>[2x]GPVHINKGGRPRQHLLSLTRRAQKHRLRELKIQVKEFADKEEGGDVKAVCLTLFLLALRARNEHRQADELEAIMQGRGSGLQPAVCLAIRVNTFLSCSQYHKMYRTVKAITGRQIFQPLHALRNAEKVLLPGYHPFEWQPPLKNVSSRTDVGIIDGLSGLASSVDEYPVDTIAKRFRYDSALVSALMDMEEDILEGMRSQDLDDYLNGPFTVVVKESCDGMGDVSEKHGSGPAVPEKAVRFSFTVMRITIEHGSQNVKVFEEPKPNSELCCKPLCLMLADESDHETLTAILSPLIAEREAMKSSELTLEMG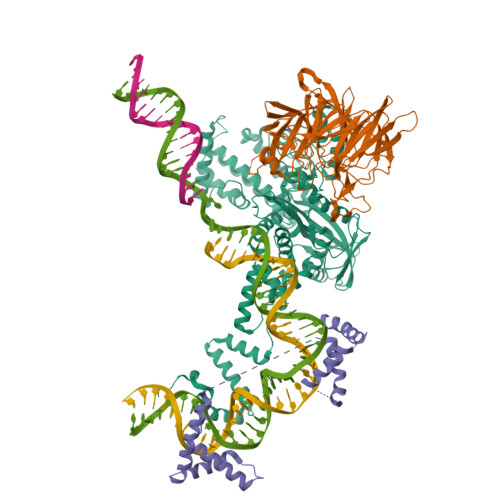GIPRTFKFIFRGTGYDEKLVREVEGLEASGSVYICTLCDTTRLEASQNLVFHSITRSHAENLQRYEVWRSNPYHESVEELRDRVKGVSAKPFIETVPSIDALHCDIGNAAEFYKIFQLEIGEVYKHPNASKEERKRWQATLDKHLRKRMNLKPIMRMNGNFARKLMTQETVDAVCELIPSEERHEALRELMDLYLKMKPVWRSSCPAKECPESLCQYSFNSQRFAELLSTKFKYRYEGKITNYFHKTLAHVPEIIERDGSIGAWASEGNESGNKLFRRFRKMNARQSKCYEMEDVLKHHWLYTSKYLQKFMNAHNA;>[2x]GPVSLQMVTVGHNIALIQPGFSLMNFDGQVFFFGQKGWPKRSCPTGVFHFDIKQNHLKLKPAIFSKDSCYLPPLRYPATCSYKGSIDSDKHQYIIHGGKTPNNELSDKIYIMSVACKNNKKVTFRCTEKDLVGDVPEPRYGHSIDVVYSRGKSMGVLFGGRSYMPSTQRTTEKWNSVADCLPHVFLIDFEFGCATSYILPELQDGLSFHVSIARNDTVYILGGHSLASNIRPANLYRIRVDLPLGTPAVNCTVLPGGISVSSAILTQTNNDEFVIVGGYQLENQKRMVCSLVSLGDNTIEISEMETPDWTSDIKHSKIWFGSNMGNGTIFLGIPGDNKQAMSEAFYFYTLRCSEEDLSEDQKIVSNSQTSTEDPGDSTPFEDSEEFCFS;> MGKGDPKKPRGKMSSYAFFVQTCREEHKKKHPDASVNFSEFSKKCSERWKTMSAKEKGKFEDMAKADKARYEREMKTYIPPKGETKKKFKDPNAPKRPPSAFFLFCSEYRPKIKGEHPGLSIGDVAKKLGEMWNNTAADDKQPYEKKAAKLKEKYEKDIAAYR N-[(cyclopentyloxy)carbonyl]-3-methyl-L-valyl-(4R)-4-[(8-bromo-7-methoxy-2-{2-[(2-methylpropanoyl)amino]-1,3-thiazol-4-yl}quinolin-4-yl)oxy]-N-[(1R,2S)-1-carboxy-2-ethenylcyclopropyl]-L-prolinamide 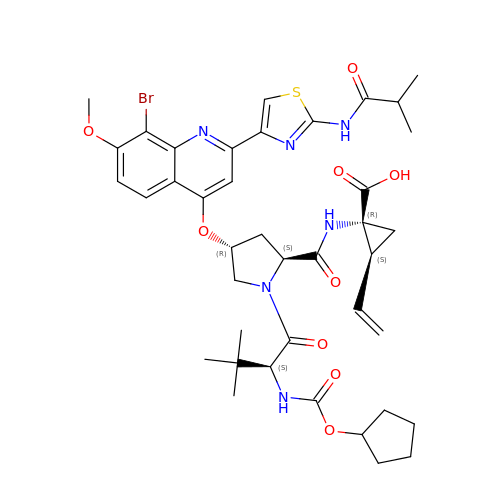| C40 H49 Br N6 O9 S | LLGDPTDZOVKFDU-XUHJSTDZSA-N> LDYHFGLE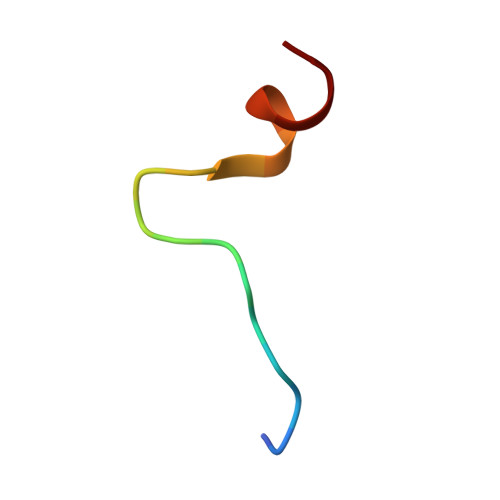EGEGIRDLFD{(3R,7S)-2-hydroxy-3-[2-(thiophen-2-yl)acetamido]-2,3,4,7-tetrahydro-1,2-oxaborepin-7-yl}acetic acid | C13 H16 B N O5 S | 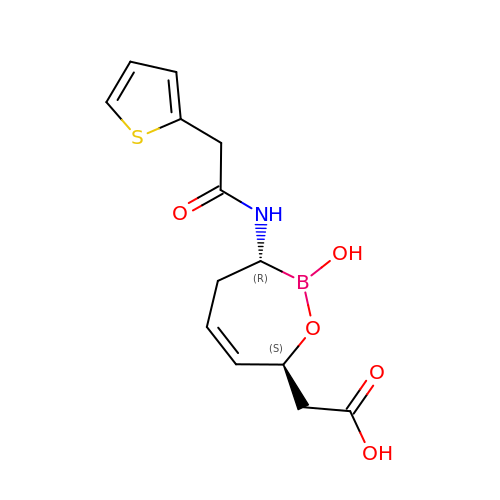JQVILEFLUQMOSI-KOLCDFICSA-N> GMALAKIVFASMTGNTEEIADIVADKLRDLGLDVDVDECTTVDASDFLEADIAIVATYTYGDGELPDEMMDFYEDLADLNLNGKIYG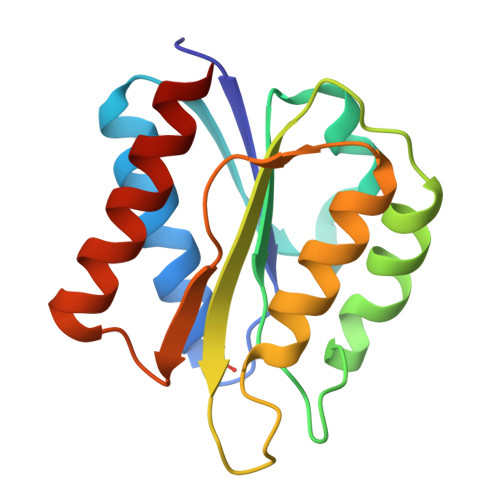VVGSGDTFYDEFCKAVDDFDRVFVSTGAEKGSECVKVDLSAEEEDIERLEQFAEELAAKVGA>[2x]MTDVIKPDYLEYDDLLDRDEMFTILEEYFMYRGLLGLRIKYGRLFNEIKKFDNDAEEQFGTIEELKQKLRLNSEEGADNFIDYIKVQKQDIVKLTVYDCISMIGLCACVVDVWRNEKLFSRWKYCLRAIKLFINDHMLDKIKSILQNRLVYVEMSKHHHHHH

Vaccinia virus, the vaccine used to eradicate smallpox, has about 200 genes, and many of these encode proteins that help the virus evade the host's immune defences. This paper concerns the vaccinia virus proteins A52 and B14, which block signalling pathways leading to the activation of the NF-κB transcription factor and thereby diminish the host immune response to infection. The structures of A52 and B14 are entirely α helical, both comprising seven α helices and adopting the Bcl-2–like fold. We show that both proteins are Bcl-2 family members but lack a surface groove for binding BH3 peptides and, consonant with this, are not anti-apoptotic. Instead these proteins have acquired the ability to inhibit signalling pathways that activate NF-κB.

A52R is an immediate-early VACV gene encoding a 23-kDa intracellular protein (A52) that contributes to virus virulence. A52 functions by inhibiting NF-κB activation downstream of the IL-1 receptor and TLRs via interactions with IRAK2 and TRAF6. The structures of two independent crystal forms of an N-terminal truncated form of A52 comprising residues 37–190 (A52ΔN36) were refined to 1.9 Å and 2.8 Å resolution with residuals R/Rfree = 0.177/0.215 and 0.181/0.192, respectively, with residues 40–189 being observed in electron density maps in both crystal forms. Residue 190 and the first two residues of the polyHis purification tag were also visible in the low-resolution structure. Both crystal forms of A52 contain 2 molecules per asymmetric unit arranged as a dimer, the overall fold (0.32±0.07 Å root-mean-squared displacement [rmsd] over 150 Cα atoms) and dimer interface being highly conserved. The final 46 residues, removed in the A52ΔC46 truncation mutant that abolished TRAF6 binding and the ability to stimulate p38 MAP kinase, comprise the final 6 residues of helix 5 and all of helices 6 and 7. Given that helices 5 and 6 contribute to the central core of the protein, it is unclear whether this truncated protein would be stable and natively folded let alone whether it would dimerise like the native protein (900 Å2 of the 1,300 Å2 of surface area buried by the native dimer interface being abolished by the truncation). Further study is therefore required to identify the binding face of TRAF6 on the surface of A52. Superposition of our structures onto that of myxoma virus M11 in complex with the BH3 peptide of Bak reveals the hydrophobic BH3-peptide binding grooves are occluded in both A52 and B14, but not in N1. Residues 92–94 and 117–122 block the groove in A52, the C-terminal ends of helices 2 and 4 being oriented closer to each other than in M11, thereby narrowing the groove significantly, and the side chains of Q93, F94 and Y118 pointing directly into and filling the groove.METHANOL TRIAZOL ETHYL PHENYL 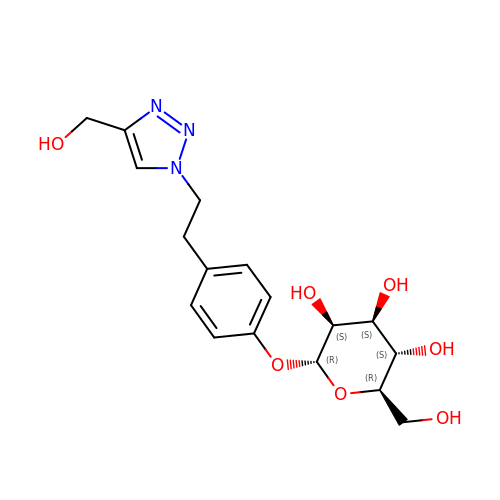1O-ALPHA-D-MANNOPYRANOSIDE | C17 H23 N3 O7 | BCFCTVRYNLVCND-NRKLIOEPSA-N>[3x]MSRKRSTKPKPAAKIALKKYNDQFLEALKLYEGKQYKKSLKLLDAILKKDGSHVDSLALKGLDLYSVGEKDDAASYVANAIRKIEGASASPICCHVLGIYMRNTKEYKESIKWF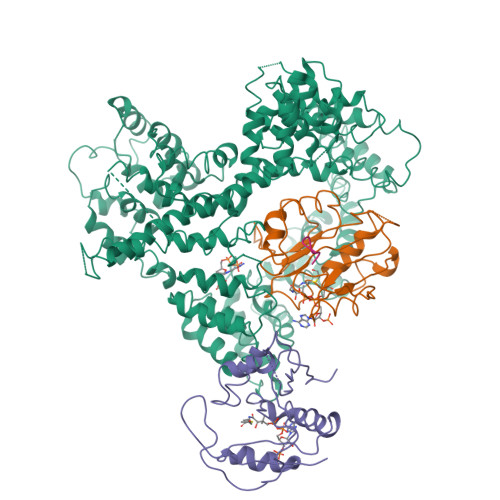TAALNNGSTNKQIYRDLATLQSQIGDFKNALVSRKKYWEAFLGYRANWTSLAVAQDVNGERQQAINTLSQFEKLAEGKISDSEKYEHSECLMYKNDIMYKAASDNQDKLQNVLKHLNDIEPCVFDKFGLLERKATIYMKLGQLKDASIVYRTLIKRNPDNFKYYKLLEVSLGIQGDNKLKKALYGKLEQFYPRCEPPKFIPLTFLQDKEELSKKLREYVLPQLERGVPATFSNVKPLYQRRKSKVSPLLEKIVLDYLSGLDPTQDPIPFIWTNYYLSQHFLFLKDFPKAQEYIDAALDHTPTLVEFYILKARILKHLGLMDTAAGILEEGRQLDLQDRFINCKTVKYFLRANNIDKAVEVASLFTKNDDSVNGIKDLHLVEASWFIVEQAEAYYRLYLDRKKKLDDLASLKKEVESDKSEQIANDIKENQWLVRKYKGLALKRFNAIPKFYKQFEDDQLDFHSYCMRKGTPRAYLEMLEWGKALYTKPMYVRAMKEASKLYFQMHDDRLKRKSDSLDENSDEIQNNGQNSSSQKKKAKKEAAAMNKRKETEAKSVAAYPSDQDNDVFGEKLIETSTPMEDFATEFYNNYSMQVREDERDYILDFEFNYRIGKLALCFASLNKFAKRFGTTSGLFGSMAIVLLHATRNDTPFDPILKKVVTKSLEKEYSENFPLNEISNNSFDWLNFYQEKFGKNDINGLLFLYRYRDDVPIGSSNLKEMIISSLSPLEPHSQNEILQYYL;>MPINIRRATINDIICMQNANLHNLPENYMMKYYMYHILSWPEASFVATTTTLDCEDSDEQDENDKLELTLDGTNDGRTIKLDPTYLAPGEKLVGYVLVKMNDDPDQQNEPPNGHITSLSVMRTYRRMGIAENLMRQALFALREVHQAEYVSLHVRQSNRAALHLYRDTLAFEVLSIEKSYYQDGEDAYAMKKVLKLEELQISNFTHRRLKENEEKLEDDLESDLLEDIIKQGVNDIIV[3x];>MGRDICTLDNVYANNLGMLTKLAHVTVPNLYQDAFFSALFAEDSLVAKNKKPSSKKDVHFTQMAYYSEIPVGGLVAKLVPKKQNELSLKGIQIEFLGVLPNYRHKSIGSKLLKFAEDKCSECHQHNVFVYLPAVDDLTKQWFIAHGFEQVGETVNNFIKGVNGDEQDAILLKKHIS[3x];>SYSMEHFR[3x]>[2x]TLHKERRIGRLSVLLLLNEAEESTQVEELERDGWKVCLGKVGSMDAHKVIAAIETASKKSGVIQSEGYRESHALYHATMEALHGVTRGEMLLGSLLRTVGL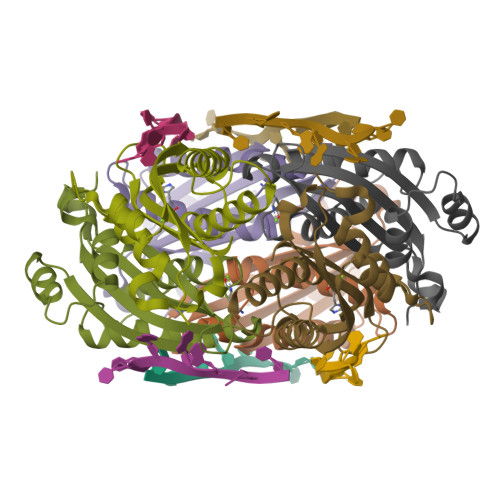RFAVLRGNPYESEAEGDWIAVSLYGTIGAPIKGLEHETFGVGINHI>MKIEDIYQFFENPPPTYLCQEVAICYILYVLLQGESYGTELIQQLETEHPTYRLSDTVLYSAIKFLEDNRAITGYWKKLEGRGRPRRMYQVSPEWQHQAEDLARLWQNYIYVRT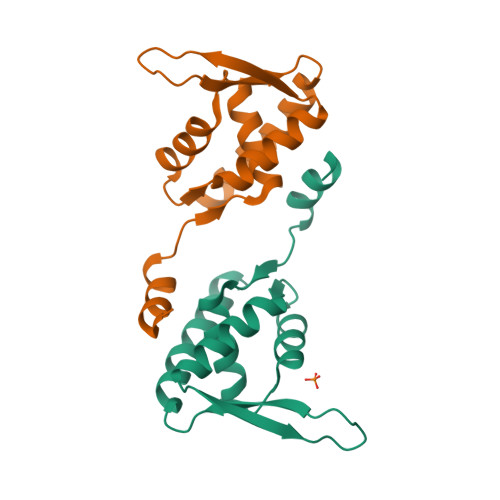N[2x]> GSMETCENVDCGPGKKCRMNKKNK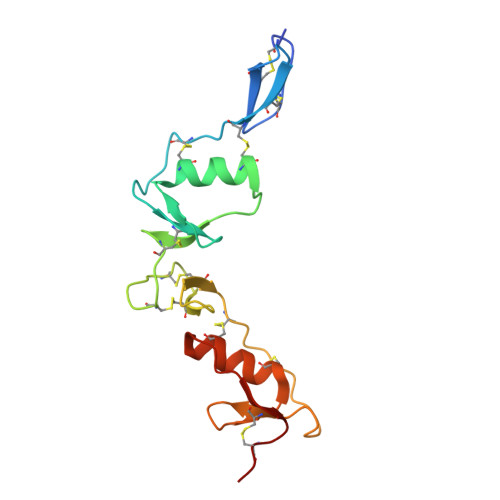PRCVCAPDCSNITWKGPVCGLDGKTYRNECALLKARCKEQPELEVQYQGKCKKTCRDVFCPGSSTCVVDQTNNAYCVTCNRICPEPSSSEQSLCGNDGVTYSSACHLRKATCLLGRSIGLAYEGKCIK Within this complex, UvrA acts as the initial damage sensor but hands off the lesion-containing DNA to UvrB and dissociates, leaving UvrB bound to the lesion in a preincision complex, the precise nature of which is not known. Both UvrA and UvrB expend ATP to form the preincision complex, which is believed to require threading of a β-hairpin element on UvrB through the DNA duplex. UvrB presents the lesion-containing strand to UvrC, which catalyzes hydrolysis of the 5th phosphodiester bond 3′ to the lesion and then the 8th phosphodiester bond 5′ to the lesion. UvrB is classified as a member of SF2 helicases on the basis of conserved helicase motifs (I-VI) (Supplementary ).

We therefore introduced a mutant Cys residue into the hydrophobic pocket and disulfide-crosslinked the resulting UvrB(T251C) protein to a single-stranded DNA substrate containing a thiol-tethered nucleobase, a cytosine. The complimentary strand is designed to contain two pyrimidine-pyrimidine mismatches on the immediate 5′ side of the modified cytosine; these were introduced to destabilize the duplex in the region expected to form a bubble, thereby facilitating maintenance of the helix-penetrated state for the β-hairpin. We determined crystal structures of UvrB disulfide-crosslinked to a 20-mer duplex substrate, in both the presence and absence of ATP, at 2.6 Å and 2.8 Å resolution, respectively. As expected on the basis of the synthetic crystallography approach used to trap these structures, the 13th nucleobase on the inner strand, a cytosine, is extruded from the duplex and inserted into the hydrophobic pocket between domains 1a and 1b. As predicted, in our structures the β-hairpin loop was found to be fully inserted between the two DNA strands, clamping the inner strand between the β-hairpin and domain 1b (Figures 3a–3(c)). Though insertion of the β-hairpin loop requires disruption of only one or two base-pairs at the insertion site, our structures reveal disruption of base-pairing throughout the entire 6 bp duplex region comprising the crosslinked cytosine. Previous DNA-bound structures of UvrB bore only fragmentary nucleic acids, leaving uncertain the overall disposition of the DNA duplex with respect to the protein. In our structures of a lesion-mimetic recognition complex, the duplex runs along the entire long axis of UvrB, contacting every domain except for domain 2 (Figures 3a–3(c)). The outer strand also makes contacts to UvrB, but these comprise almost exclusively van der Waals interactions. In agreement with previous EM studies, the UvrB-bound DNA contains a sharp bend (~60°) localized at the junction between the bubble and the fully base-paired segment flanking on its left side (“left flank,” Figure 3d). If so, the observed contacts between the helicase motifs engaged in DNA binding and the inner strand phosphates suggest that our structures obtained in both the presence and absence of ATP (hydrolyzed to ADP and Pi in crystallo) represent “open” states.

>VEGRFQLVAPYEPQGDQPQAIAKLVDGLRRGVKHQTLLGATGTGKTFTISNVIAQVNKPTLVIAHNKTLAGQLYSELKEFFPHNAVEYFVSYYDYYQPEAYVPQTDTYIEKDAKINDEIDKLRHSATSALFERRDVIIVASVSSIYGLGSPEEYRELVVSLRVGMEIERNALLRRLVDIQYDRNDIDFRRGTFRVRGDVVEIFPASRDEHSIRVEFFGDEIERIREVDALTGEVLGEREHVAIFPASHFVCREEKMRLAIQNIEQELEERLAELRAQGKLLEAQRLEQRTRYDLEMMREMGFSSGIENYSRHLALRPPGSTPYTLLDYFPDDFLIIVDESHVTLPQLRGMYNGDRARKQVLVDHGFRLPSALDNRPLTFEEFEQKINQIIYVSATPGPYELEHSPGVVEQIIRPTGLLDPTIDVRPTKGQIDDLIGEIRERVERNERTLVTTLTKKMAEDLTDYLKEAGIKVAYLHSEIKTLERIEIIRDLRLGKYDVLVGINLLREGLDIPEVSLVAILDADKEGFLRSERSLIQTIGRAARNANGHVIMYADTITKSMEIAIQETKRRRAIQEEYNRKHGIVPRTVKKEIR[2x]>[4x]VSEDLRSRIEVLKRKVIEKVQHIQLLQKNVRAQLVDMKRLEVDIDIKIRSCRGSCSRALAREVDLKDYEDQQKQLEQVIAKDLLPSR;>[4x]DNENVVNEYSSELEKHQLYIDETVNSNIPTNLRVLRSILENLRSKIQKLESDVSAQMEYCRTPCTVSCNIPVVSGKECEEIIRKGGETSEMYLIQPDSSVKPYRVYCDMNTENGGWTVIQNRQDGSVDFGRKWDPYKQGFGNVATNTDGKNYCGLPGEYWLGNDKISQ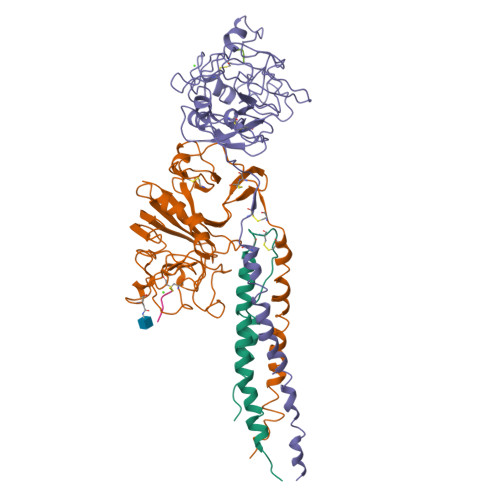LTRMGPTELLIEMEDWKGDKVKAHYGGFTVQNEANKYQISVNKYRGTAGNALMDGASQLMGENRTMTIHNGMFFSTYDRDNDGWLTSDPRKQCSKEDGGGWWYNRCHAANPNGRYYWGGQYTWDMAKHGTDDGVVWMNWKGSWYSMRKMSMKIRPFFPQQ;>[4x]MLEEIMKYEASILTHDSSIRYLQEIYNSNNQKIVNLKEKVAQLEAQCQEPCKDTVQIHDITGKDCQDIANKGAKQSGLYFIKPLKANQQFLVYCEIDGSGNGWTVFQKRLDGSVDFKKNWIQYKEGFGHLSPTGTTEFWLGNEKIHLISTQSAIPYALRVELEDWNGRTSTADYAMFKVGPEADKYRLTYAYFAGGDAGDAFDGFDFGDDPSDKFFTSHNGMQFSTWDNDNDKFEGNCAEQDGSGWWMNKCHAGHLNGVYYQGGTYSKASTPNGYDNGIIWATWKTRWYSMKKTTMKIIPFNRLTIGEGQQHHLGGAKQAGDV;>[8x]GPRPX N-tert-butyl-1-(1-{5-[5-(trifluoromethyl)-1,3,4-oxadiazol-2-yl]pyridin-2-yl}piperidin-4-yl)-1H-imidazole-5-carboxamide 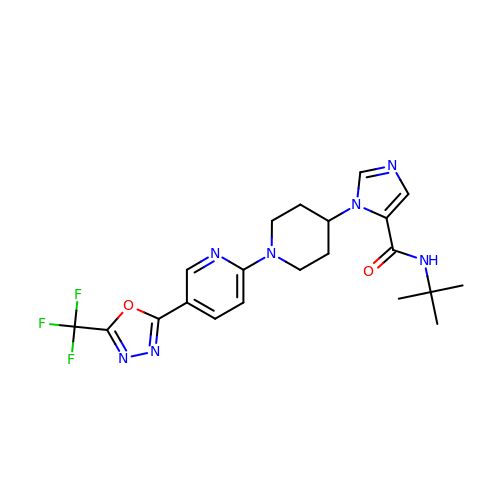| C21 H24 F3 N7 O2 | HWSHOMMVLGBIDN-UHFFFAOYSA-N> IQPPPVNRNL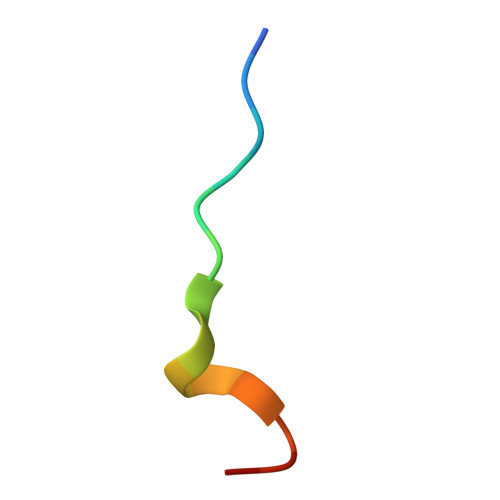KPDRK>MERQNIHNFGAGPAAMAKEVIEATAKAVNNFWEGLSILEISHRSKEWINVMNETKALMKEVMDIPEGYEILFFGGGASLQFLMVAMNLLNKKACYLDTGVWASKAIKEAENIGEVKIIGTSKDKNYTYIPEYQIPSDYDYFHITTNNTIYGTEIRKDIESPIPLVADMSSDILSKPIDISKYSLIYAGAQKNCGAAGVTIVIIKKEILGKVQRKIPIILDYQVHILNNSMYNTPPVISIFTVNQTLKYIKKIGGLKKIQELNEEKARLLYAEIDRNKIFRGTVRKKDRSIMNVCFVMEEQYKQLENEFSEYALQKGIIGIKGHRSV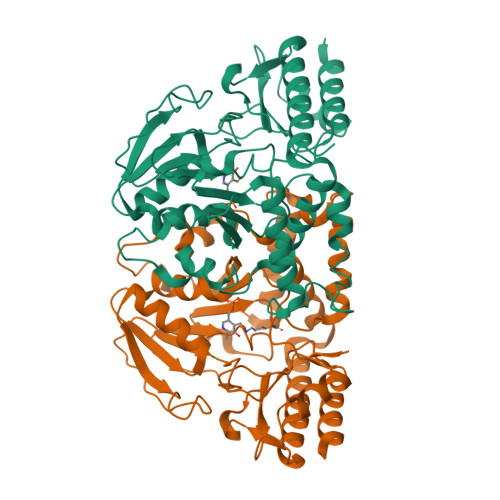GGFRASIYNAVTIESVQALIKCMHDFEQLHTH[12x]Cables formed by head-to-tail polymerization of tropomyosin, localized along the length of sarcomeric and cytoskeletal actin filaments, play a key role in regulating a wide range of motile and contractile processes. Here, we present high–resolution structures of cables formed by acetylated and unacetylated Schizosaccharomyces pombe tropomyosin ortholog TpmCdc8. All homodimer conformers are approximately 230 Å in length and exhibit head–to–tail interactions, where the N–termini of one homodimer contact the C–termini of an adjacent homodimer. Each of the conformers that make up the TpmCdc8 cables consists of two α-helices that are wrapped around each other, forming a left-handed coiled–coil structure.

Despite the high similarity of space group and unit cell parameters with the structure of the unacetylated protein in space group P1, solving the structure of acetylated TpmCdc8 by molecular replacement using regions of the unacetylated structure as search models repeatedly failed. We were able to solve this structure by molecular replacement of ideal helical fragments using the coiled-coil mode of ARCIMBOLDO-LITE. N-terminal acetylation of TpmCdc8 induces structural changes that result in a different architecture of the overlap junction. The carbonyl oxygen atom of the acetyl group forms an additional hydrogen bond with the backbone nitrogen atom of residue L4 within the same helix, thereby stabilizing the helical structure at the N-terminus. Additionally, the methyl group of the acetyl group forms a hydrophobic interaction with the residues L158 and H155 of the C-terminal coiled-coil. The increased helicity triggers a change in the overall architecture of the overlap junction, with the result that the acetylated N-termini, which are less flexible, move closer together. The distance between the methionine Cα atoms of chains A and B shortens from 17.5 Å in the unacetylated structure to 12.7 Å in the acetylated structure. Key ionic interactions, stabilizing the overlap junction of conf-A1 include those between residue R12 and the C–terminus as well as residue K3, the C-terminus and residue E159. As predicted by an analysis of the B-factors of the conformer structures, conf A1 showed a narrow ensemble distribution, while those for conf-U1, conf-U2 and conf-U3 were much wider indicating increased flexibility of their overlap junctions. The acetylation therefore leads to a more energetically favorable overlap junction compared to conf-U1 and the average of all unacetylated conformers (−40.8 ± 12.79 kcal/mol).

>[2x]XMDKLREKINAARAETDEAVARAEAAEAKLKEVELQLSLKEQEYESLSRKSEAAESQLEELEEETKQLRLKADNEDIQKTEAEQLSRKVELLEEELETNDKLLRETTEKMRQTDVKAEHFERRVQSLERERDDMEQKLEEMTDKYTKVKAELDEVHQALEDL>MSRAYDLVVIGAGSGGLEAGWNAASLHKKRVAVIDLQKHHGPPHYAALGGTCVNVGCVPKKLMVTGANYMDTIRESAGFGWELDRESVRPNWKALIAAKNKAVSGINDSYEGMFADTEGLTFHQGWGALQDNHTVLVRESADPNSAVLETLDTEYILLATGSWPQHLGIEGDDLCITSNEAFYLDEAPKRALCVGGGYISIEFAGIFNAYKARGGQVDLAYRGDMILRGFDSELRKQLTEQLRANGINVRTHENPAKVTKNADGTRHVVFESGAEADYDVVMLAIGRVPRSQTLQLDKAGVEVAKNGAIKVDAYSKTNVDNIYAIGDVTDRVMLTPVAINEGAAFVDTVFANKPRATDHTKVACAVFSIPPMGVCGYVEEDAAKKYDQVAVYESSFTPLMHNISGSTYKKFMVRIVTNHA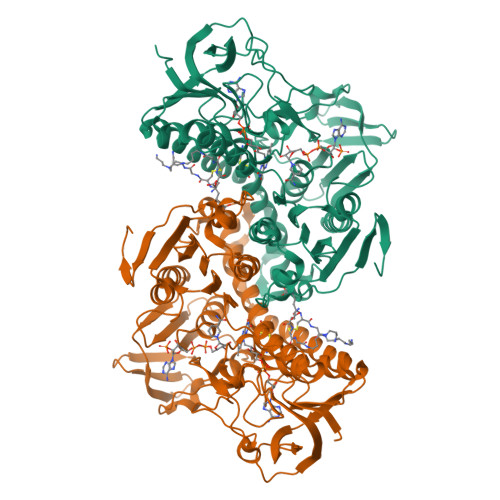DGEVLGVHMLGDSSPEIIQSVAICLKMGAKISDFYNTIGVHPTSAEELCSMRTPAYFYQKGKRVEKI[2x]>GSHMATVQQLEGRWRLVDSKGFDEYMKELGVGI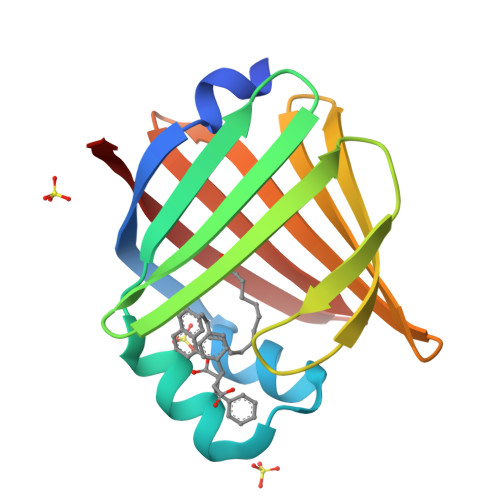ALRKMGAMAKPDCIITCDGKNLTIKTESTLKTTQFSCTLGEKFEETTADGRKTQTVCNFTDGALVQHQEWDGKESTITRKLKDGKLVVECVMNNVTCTRIYEKVE[8x]>[4x]GPGSMSLKVNILGHEFSNPFMNAAGVLCTTEEDLRRMTESESGSLIGKSCTLAPRTGNPEPRYFGLPLGSINSMGLPNLGVDFYLSYAAQTHDYSRKPLFLSMSGLSVEESVEMVKKLVPITKEKGTILEL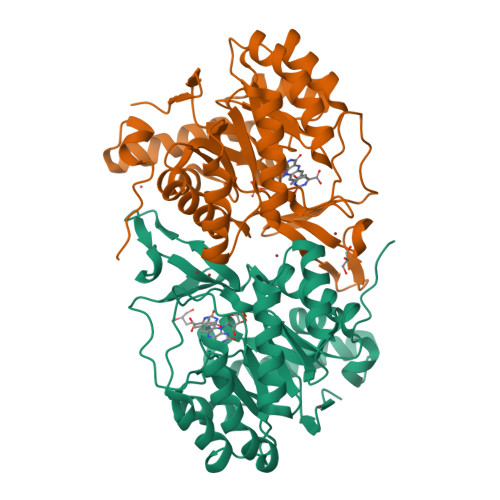NLSCPNVPGKPQVGYDFDTTRTYLQKVSEAYGLPFGVKMPPYFDIAHFDMAAAVLNDFPLVKFITCVNSIGNGLVIDPANETVVIKPKQGFGGLGGKYVLPTALANVNAFFRRCPDKLVFGCGGVYSGEEAFLHILAGASMVQVGTALHDEGPIIFARLNKELQEIMTNKGYKTLDEFRGRVKTMD>[20x]MKYVVVSGGVISGIGKGVLASSTGMLLKTLGLKVTSIKIDPYMNIDAGTMSPLEHGECFVLDDGGETDLDLGNYERYLGITLSRDHNITTGKIYSHVISRERRGDYLGKTVQIVPHLTNAIQDWIQRVSKIPVDDTGLEPDVCIIELGGTVGDIESAPFVEALRQFQFEVGRENFALIHVSLVPVIHGEQKTKPTQAAIKDLRSLGLIPDMIACRCSEELNRSTIDKIAMFCHVGPEQVVNVHDVNSTYHVPLLLLKQHMID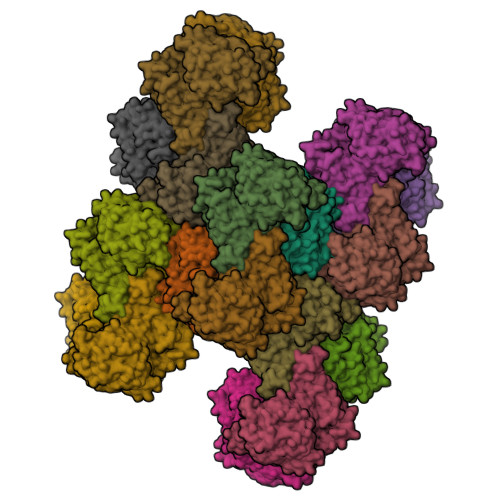YLHSRLKLGEVPLTLEDKERGSQLLTNWENMTKNLDDSDDVVKIALVGKYTNLKDSYLSVTKSLEHASMKCRRQLEILWVEASNLEPETQEVDKNKFHDSWNKLSSADGILVPGGFGTRGIEGMILAAKWARESGVPFLGVCLGLQVAAIEFARNVIGRPNSSSTEFLDETLLAPEDQVVITMRLGLRPTIFQPNSEWSNIRKLYGEVNEVHERHRHRYEINPKIVNDMESRGFIFVGKDETGQRCEIFELKGHPYYVGTQYHPEYTSKVLEPSRPFWGLVAAASGTLGEVIKDINL1-(2,6-difluorophenyl)-3-[[3-[5-hydroxy-4-(1H-pyrrolo[3,2-c]pyridin-2-yl)pyrazol-1-yl]phenyl]methyl]urea 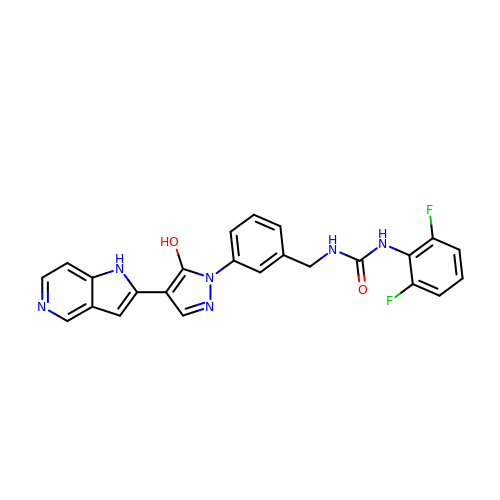| C24 H18 F2 N6 O2 | BWWQOZHMBUJBOQ-UHFFFAOYSA-N>GDDSVLKVGASPVPHAEILEHVKPLLEKEGVKLEVTTYTDYVLPNKALESGDIDANYFQHVPFFNEAVKENDYDFVNAGAIHLEPVGLYSKKYKSLQEIPDGSTIYVSSSVSDWPRVLTILEDAGLITLKEGVDRTTATFDDIDKNTKKLKF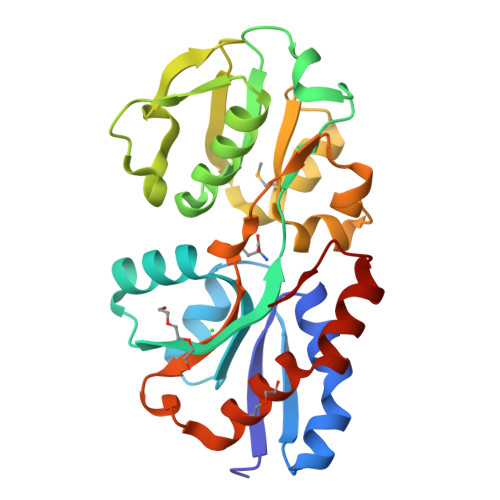NHESDPAIMTTLYDNEEGAAVLINSNFAVDQGLNPKKDAIALEKESSPYANIIAVRKEDENNENVKKLVKVLRSKEVQDWITKKWNGAIVPVNE[2x]>MALLTPIPSPMVNLTQVIDPTEQLAYFPKITFERLKNYDTSSNYAKGKLTRNYMILLPWQHVNRYNFVFSSTGCKVSLKTCIGKLMKDLNPKVLYFIGEGAGNWMARTACEYPDIKFVYRSLKDDLDHHYPLEYQRVIGELSRIIDSGEGLSMETTDATQKTHWDLIHRVSKDALLITLCDAEFKDRDDFFKMVILWRKHVLSCRICTTYGTDLYLFAKYHAKDCNVKLPFFVRSVATFIMQGSKLSGSECYILLTLGHHNNLPCHGEIQNSKMKIAVCNDFYAAKKLDNKSIEANCKSLLSGLRIPINKKELNRQRRLLTLQSNHSSVATVGGSKVIESKWLTNKANTIIDWLEHILNSPKGELNYDFFEALENTYPNMIKLIDNLGNAEIKKLIEVTGYMLVSKKSGHHHHHH[2x]

The Mononegavirales order groups five families of monopartite, negative-strand RNA viruses many of which are highly pathogenic and/or contagious; the Filoviridae (of which Ebola virus is a representative), the Bornaviridae (Borna disease virus), the Nyamiviridae (midway virus), the Rhabdoviridae (rabies, vesicular stomatitis virus (VSV)) and the Paramyxoviridae (measles virus, human metapneumovirus (hMPV)). These viruses encode a large RNA polymerase (L) (usually >2,000 amino acids) that is crucial to viral replication. As a part of this study, we expressed CR-VI+, a 406-residue fragment comprising CR-VI and the adjoining ‘+ domain’, the variable region carrying the K-K-G-motif, investigated its MTase activity and solved its crystal structure. Besides sequentially methylating the 2′O and N7 atoms of small capped RNAs, CR-VI+ also 2′O methylates uncapped substrates and displays nucleotide triphosphatase (NTPase) activity. Both the CR-VI domain, which assumes a fairly standard MTase fold, and the K-K-G motif of the (mainly helical) +domain are required for the MTase reactions.

Most notably, hMPV and flaviviruses share an unusually long (∼10 residues), flexible β2λ (that is, the loop immediately following the β2-strand), which forms the SAM-binding pocket (SAMP) along with loops β1λ and β4λ, shielding it from the solvent. In CR-VI+, β2λ similarly assumes alternate conformations. In the ‘closed’ form, the ligand’s ribose group is hydrogen bonded to D1725, and—via a water—to D1722. Loops β1λ and β4λ also show a degree of flexibility. β1λ residue E1697, conserved in paramyxo- and filoviruses, forms a hydrogen bond with the NH2 group of SAM and is essential for both MTase activities.>[2x]MGSSHHHHHHSQDPNSMTTLTRQDLNFGQVVADVLCEFLEVAVHLILYVREVYPVGIFQKRKKYNVPVQMSCH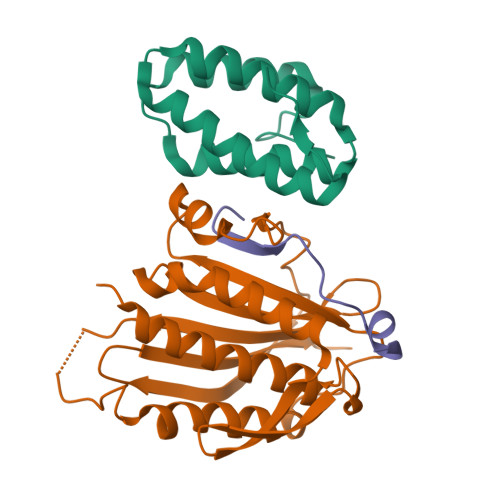PELNQYIQDTLHCVKPLLEKNDVEKVVVVILDKEHRPVEKFVFEITQPPLLSISSDSLLSHVEQLLAAFILKISVCDAVLDHNPPGCTFTVLVHTREAATRNMEKIQVIKDFPWILADEQDVHMHDPRLIPLKTMTSDILKMQLYVEERAHKGSGSGSGSGSGSH;>[2x]MLTPTPDSSPRSTSSPSQSKNGSFTPRTANILKPLMSPPSREEIMATLLDHD;>[2x]MLKHEGPPAEKPLEELSASTSGVPGLSSLQSDPAGCVRPPAPNLAGAVEFNDVKTLLREWITTISDPMEEDILQVVKYCTDLIEEKDLEKLDLVIKYMKRLMQQSVESVWNMAFDFILDNVQVVLQQTYGSTLKVT> MGGMEFIGRVVSNRMQKTVVVAVSYVVWVPKYKVYQKRVARHKARDESQASVIGDIVRIRKSRKFSREVSYSVVDTLRKAHVYDPAAAAALVATRD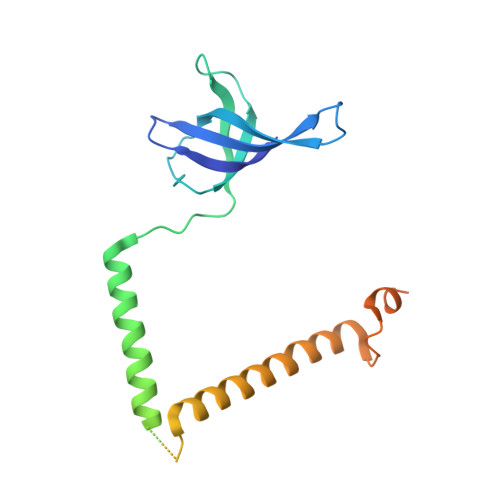AARAAAAASTGTRAGAAAAGEGQAAQLEGAGFAASGVATSSAGGRSDPWVAEAARRLDASAARLAALRELYEKEVGPGVPLSGAVLAVANSGPGGTGSVRGKAAAAAAGAAEGPGDAKAQQDKQ> MLLNPTKRERKENYSIDNYYKDVLNTGRSSTPSHPRMPKPHVFHSHQLQPPQLQVLYEKERMWTAKKTGYVPTMDDVKAAYGKISDQEEQKEKLELLKLSVNNSQPLTEEEEKMKADWESEGFTNWNKLEFRKFITVSGKYGRNSIQAIARELAPGKTLEEVRAYAKAFWSNIERIEDYEKYLKIIENEEEKIKRVKMQQEALRRKLSEYKNPFFDLKLKHPPSSNNKRTYSEEEDRFILLMLFKYGLDRDDVYELVRDEIRDCPLFELDFYFRSRTPVELARRGNTLLQCLEKEFNAGIVLDD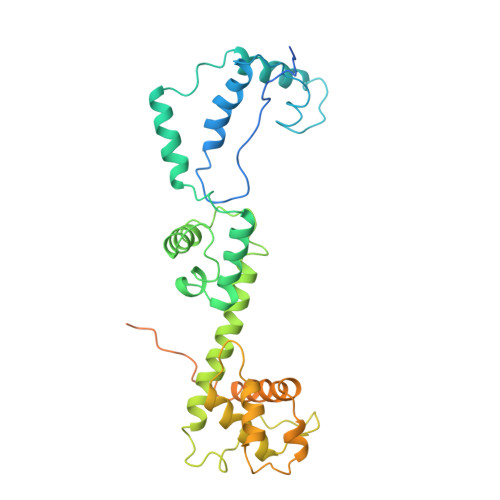ATKDRMKKEDENGKRIREEFADQTANEKENVDGVESKKAKIEDTSNVGTEQLVAEKIPENETTHHHHHHH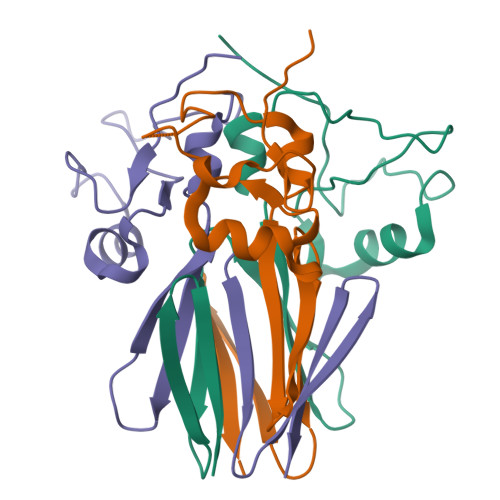>[3x]NNTPVTNKLKAYGDANFNFTNNSIADAEKQVQEAYKGLLNLNEKNASDKLLVEDNTAATVGNLRKLGWVLSSKNGTRNEKSQQVKHADEVLFEGKGGVQVTSTSENGKHTITFALA>MRPETIPGISLNEDNSHYFYTRAGRRLSAEEVDSWVDQYAGTQVKELMLCPNCMRTSYASQVWDPIWRGYDPAGPDDQPLLASLPPEERVAARGWIHTAWQLHQDGIDIYARWIRRCRQRGISPWISMRMNDVHYVNDERCFLHSEFWRENPQLRRVPYRFAEWTDRAFDYGRAEVREHHLKLIRELAARYDFDGLELDWMRFGFHFRPGYEAEGAEILTAFTAEVRRLLDDWEKRRGHKIHLGARIPSRPATALGLGMDAVTWARRGLVDMLVITPFWASAETDMPVEIWRQLLEGTGVTLAAGLEVLLRPYPDSPLFQTNSLETVRGAAASLLDRGAQRIYLFNYMDSQTAMEDLENYPTLLREIGSLETLAGKPRRHVLTFADTWAPGEPRAIPLPATCRPGEWRAFRLHTGPKPEPGEVIAALGIEGGVAIGPETLEVRVNGELC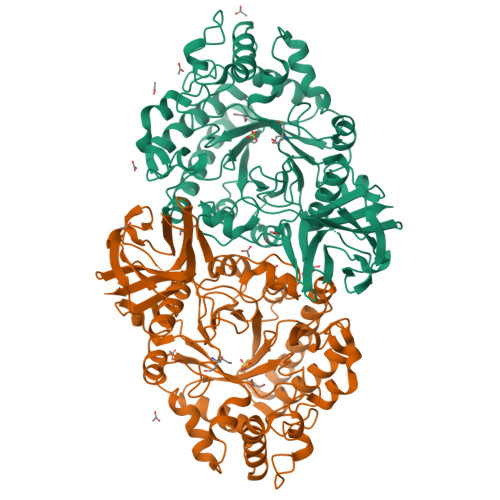AFLGLVDLSKPRPDFPVYGFSVPLAAMRRGYNLIEVTARQELRFGWAEFLIRPWHSHHHHHH[2x]> RNCSSNEERKRRKYFHMLYLVCLMVHGFIRNEWINSKRLSRKLSNLVPEKVFELLHPQKDEELPLRSTRKLLDGLKKCMELWQKHWKITKKYDNEGLYMRTWKEIEMSANNKRKFKTLKRSDFLRAVSKGHGDPDIS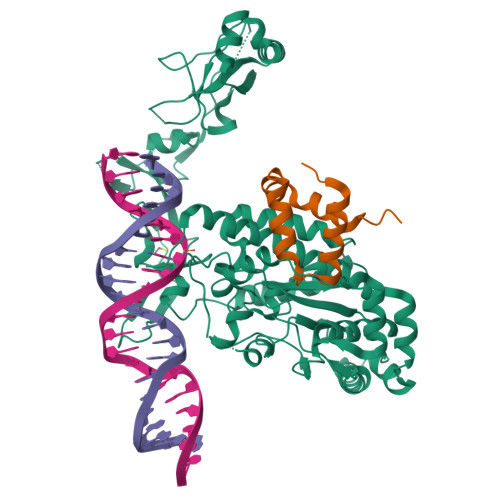VQGFVAMLRACNVNARLIMSCQPPDFTNMKIDTSLNGNNAYKDMVKYPIFWCEVWDKFSKKWITVDPVNLKTIEQVRLHSKLAPKGVACCERNMLRYVIAYDRKYGCRDVTRRYAQWMNSKVRKRRITKDDFGEKWFRKVITALHHRKRTKIDDYEDQYFFRRDESEGIPDSVQDLKNHPYYVLEQDIKQTQIVKPGCKECGYLKVHGKVGKVLKVYAKRDIADLKSARQWYMNGRILKTGSRCKKVIKRTVGRPKGEAEEDAERLYSFEDTELYIPPLASASGEITKNTFGNIEVFAPTMIPGNCCLVENPVAIKAARFLGVEFAPAVTSFKFERGSTVKPVLSGIVVAKWLREAIETAIDGIEFI;> AGLTVEDLLSLRQVVSGNPEALAPLLENISARYPQLREHIMANPEVFVSMLLEAVGD> VDYAPAQAQIVHAGQACVVKEDNISERVYTIREGDTLMLQCLVTGHPRPQVRWTKTAGSASDKFQETSVFNETLRIERIARTQGG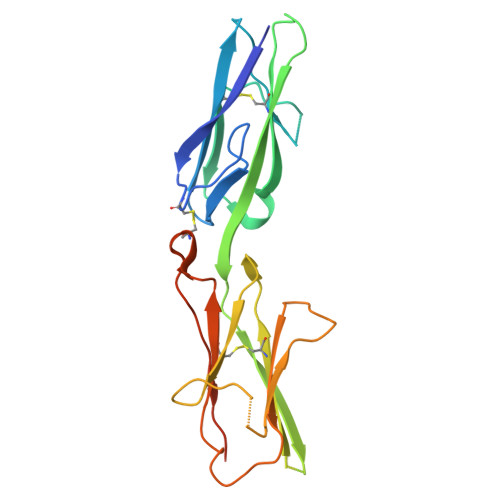RYYCKAENGVGVPAIKSIRVDVQYLDEPMLTVHQTVSDVRGNFYQEKTVFLRCTVNSNPPARFIWKRGSDTLSHSQDNGVDIYEPLYTQGETKVLKLKNLRPQDYASYTCQVSVRNVCGIPDKAITFRLTNTTGSASTSHHHHHH> MFAQEALTTQYSQSELLKNWALSHCLALVYKDDVVKNDARATASAYLEYGKQSVEIYHEIDEIAKKYSGLKYNGS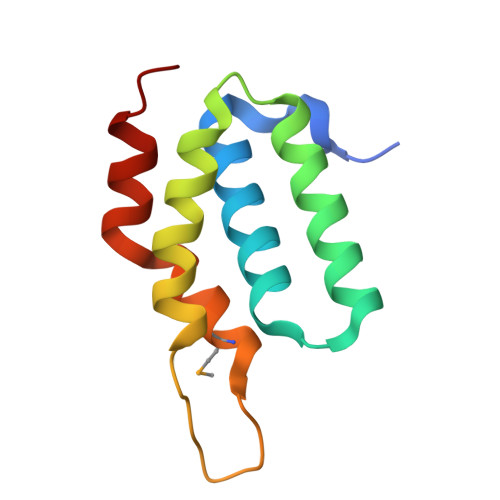ISSDFNTMKCIDFIHDRELNELIKRRVEK> MATEHPEPPKAELQLPPPPPPGHYGAWAAQELQAKLAEIGAPIQGNREELVERLQSYTRQTGIVLNRPVLRGEDGDKAAPPPMSAQLPGIPMPPPPLGLPPLQPPPPPPPPPPGLG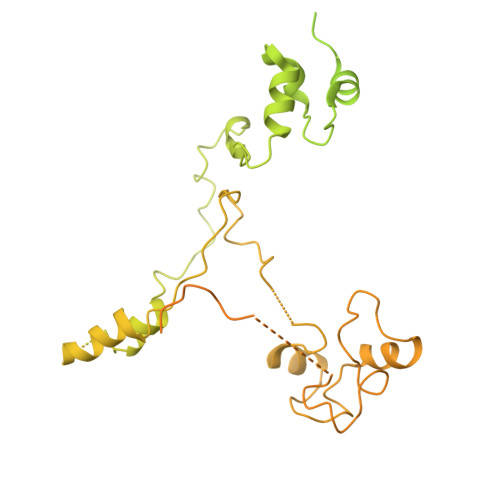LGFPMAHPPNLGPPPPLRVGEPVALSEEERLKLAQQQAALLMQQEERAKQQGDHSLKEHELLEQQKRAAVLLEQERQQEIAKMGTPVPRPPQDMGQIGVRTPLGPRVAAPVGPVGPTPTVLPMGAPVPRPRGPPPPPGDENREMDDPSVGPKIPQALEKILQLKESRQEEMNSQQEEEEMETDARSSLGQSASETEEDTVSVSKKEKNRKRRNRKKKKKPQRVRGVSSESSGDREKDSTRSRGSDSPAADVEIEYVTEEPEIYEPNFIFFKRIFEAFKLTDDVKKEKEKEPEKLDKLENSAAPKKKGFEEEHKDSDDDSSDDEQEKKPEAPKLSKKKLRRMNRFTVAELKQLVARPDVVEMHDVTAQDPKLLVHLKATRNSVPVPRHWCFKRKYLQGKRGIEKPPFELPDFIKRTGIQEMREALQEKEEQKTMKSKMREKVRPKMGKIDIDYQKLHDAFFKWQTKPKLTIHGDLYYEGKEFETRLKEKKPGDLSDELRISLGMPVGPNAHKVPPPWLIAMQRYGPPPSYPNLKIPGLNSPIPESCSFGYHAGGWGKPPVDETGKPLYGDVFGTNAAEFQTKTEEEEIDRTPWGELEPSDEESSEEEEEEESDEDKPDETGFITPADSGLITPGGFSSVPAGMETPELIELRKKKIEEAMDGSETPQLFTVLPEKRTATVGGAMMGSTHIYDMSTVMSRKGPAPELQGVEVALAPEELELDPMAMTQKYEEHVREQQAQVEKEDFSDMVAEHAAKQKQKKRKAQPQDSRGGSKKYKEFKF>[2x]QAQITGRPEWIWLALGTALMGLGTLYFLVKGMGVSDPDAKKFYAITTL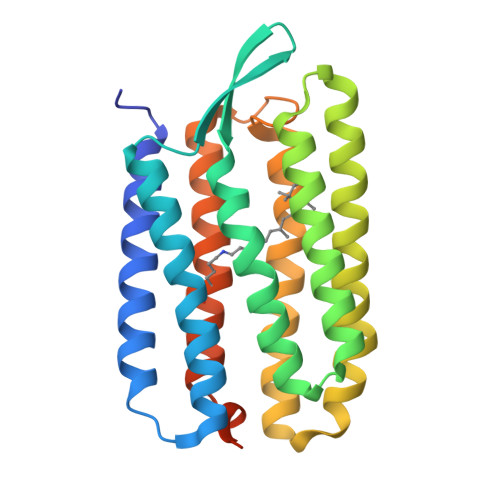VPAIAFTMYLSMLLGYGLTMVPFGGEQNPIYWARYADWLFTTPLLLLDLALLVDADQGTILALVGADGIMIGTGLVGALTKVYSYRFVWWAISTAAMLYILYVLFFGFTSKAESMRPEVASTFKVLRNVTVVLWSAYPVVWLIGSEGAGIVPLNIETLLFMVLDVSAKVGFGLILLRSRAIFGEAEAPEPSAGDGAAATSD>[2x]MSSQVEHPAGGYKKLFETVEELSSPLTAHVTGRIPLWLTGSLLRCGPGLFEVGSEPFYHLFDGQALLHKFDFKEGHVTYHRRFIRTDAYVRAMTEKRIVITEFGTCAFPDPCKNIFSRFFSYFRGVEVTDNALVNIYPVGEDYYACTETNFITKVNPETLETIKQVDLCNYVSVNGATAHPHIENDGTVYNIGNCFGKNFSIAYNIVKIPPLQADKEDPISKSEIVVQFPCSDRFKPSYVHSFGLTPNYIVFVETPVKINLFKFLSSWSLWGANYMDCFESNETMGVWLHIADKKRKKYINNKYRTSPFNLFHHINTYEDHEFLIVDLCCWKGFEFVYNYLYLANLRENWEEVKKNARKAPQPE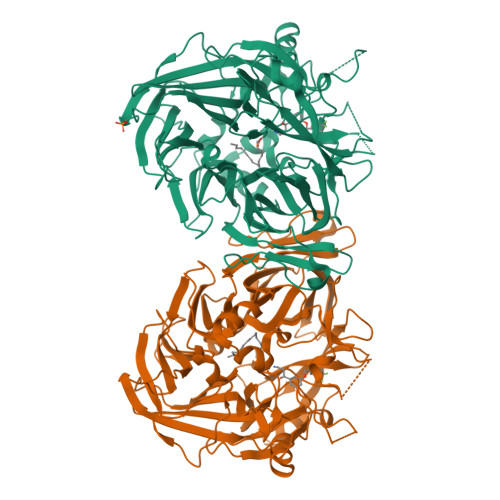VRRYVLPLNIDKADTGKNLVTLPNTTATAILCSDETIWLEPEVLFSGPRQAFEFPQINYQKYGGKPYTYAYGLGLNHFVPDRLCKLNVKTKETWVWQEPDSYPSEPIFVSHPDALEEDDGVVLSVVVSPGAGQKPAYLLILNAKDLSEVARAEVEINIPVTFHGLFKKS> GASKQSASGTIEVISRENGSGTRGAFTEITGILKKDGDKKIDNTAKTAVIQNSTEGVLSAVQGNANAIGYISLGSLTKSVKALEIDGVKASRDTVLDGEYPLQRPFNIVWSSNLSKLGQDFISFIHSKQGQQVVTDNKFIEAKTETTEYTSQ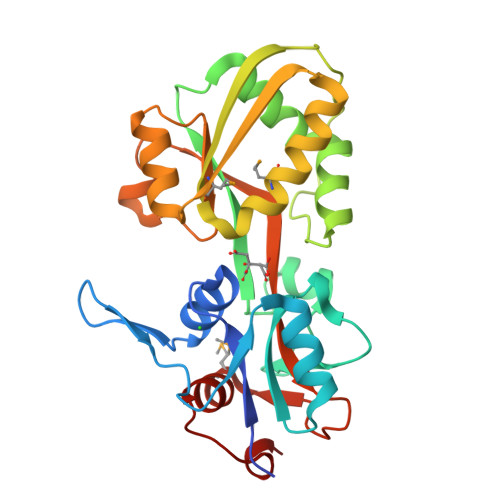HLSGKLSVVGSTSVSSLMEKLAEAYKKENPEVTIDITSNGSSAGITAVKEKTADIGMVSRELTPEEGKSLTHDAIALDGIAVVVNNDNKASQVSMAELADVFSGKLTTWDKIK>[8x]MAHHHHHHMSKPTQQGITFSKNDVEIIARETLYRGFFSLDLYRFRHRLFNGGMSG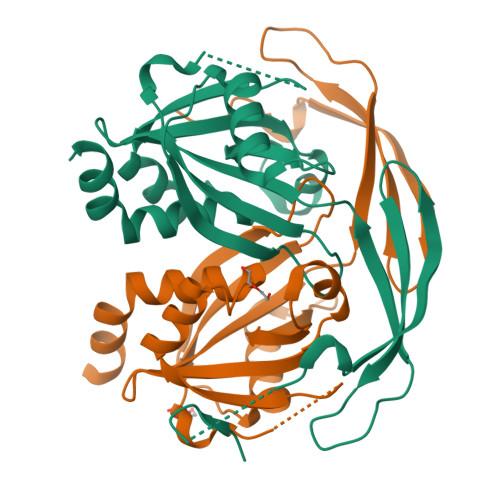EITREIFERGHAAVLLPFDPVRDEVVLVEQIRIAAYDTSESPWLLEMVAGMIEAGETVEDVARREALEEAGLEVGRTKPILSYLASPGGTSERLSILVGEVDASTAKGIHGLAEENEDIRVHVVSREQAYQWVEEGKIDNAASVIALQWLQLHYHNLRNEWTK>[2x]GSFPSTVKNGLSKIGIPSNVLDFMFDWTGSDQDYPKVPEAKGSIQAVRNEAFFIPLYELFLTYGGIFRLTFGPKSFLIVSDPSIAKHILKDNAKAYSKGILAEILDFVMGKGLIPADGEIWRRRRRAIVPALHQKYVAAMISLFGEASDRLCQKLDAAALKGEEVEMESLFSRLTLDIIGKAVFNYDFDSLTNDTGVIEAVYTVLREAEDRSVSPIPVWDIPIWKDISPRQRKVATSLKLINDTLDDLIATCKRMVEEEELQFHEEYMNERDPSILHFLLASGDDVSSKQLRDDLMTMLIAGHETSAAVLTWTFYLLTTEPSVVAKLQEEVDSVIGDRFPTIQDMKKLKYTTRVMNESLRLYPQPPVLIRRSIDNDILGEYPIKRGEDIFISVW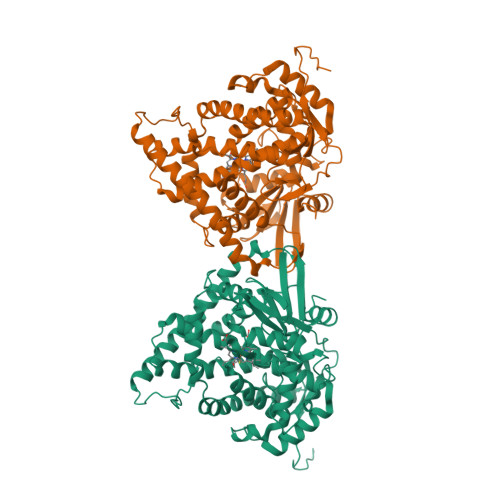NLHRSPLHWDDAEKFNPERWPLDGPNPNETNQNFSYLPFGGGPRKCIGDMFASFENVVAIAMLIRRFNFQIAPGAPPVKMTTGATIHTTEGLKLTVTKRTKPLDIPSVPILPMDTSRDEVSSALS> QFRAIIESPEGAGHVGYQYRRNTGSTMRMVSDVLDERVSLWDFHCDPSGNVIQPGPNVDSRQYLQAAIDYVSSNGGGTITIPAGYTWYLGSYGVGGIAGHSGIIQLRSNVNLNIEGRIHLSPFFDLKPFQVFVGFDNGDPASSGNLENCHIYGHGVVDFGGYEFGASSQLRNGVAFGRSYNCSVTGITFQNGDVTWAITLGWNGYGSNCYVRKCRFINLVNSSVNADHSTVYVNCPYSGVESCYFSMSSSFARNIACSVQLHQHDTFYRGSTVNGYCRGAYVVMHAAEAAGAGSYAYNMQVENNIAVIYGQFVILGSDVTATVSGHLNDVIVSGNIVSIGERAAFSAPFGAFIDIGPDNSGASNVQDIQRVLVTGNSFYAPANITDSAAITLRANLNGCTFIANNFDCRYMVYNAPGTTSPVVQNLVWDKSNVIGGTHANQRAGQNLFDMQFASVVNSTIEVQLSCEDLSMFSCILFPASCQLSYSKITVDSAW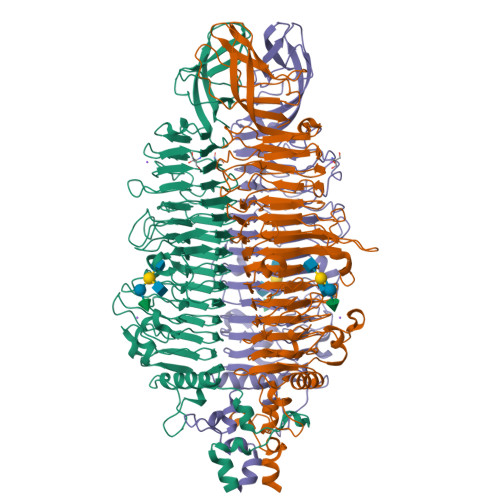TKSMSNTAVFEGNQQAGANVYVSYPATVNLTSYNTQGAVPFFSTDTNYAWVTSAYSLSINENLDFSPPATYTNKANGQLVGVGYNEIGGVRSVSVRLMLQRQV>TFRQQTIDFLNDNIRRGIENYYDDLDFK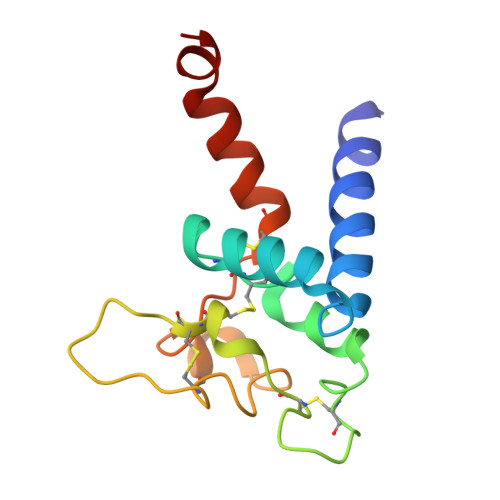NIMDFVQKKFKCCGGEDYRDWSKNQYHDCSAPGPLACGVPYTCCIRDTTEVVNTMCGYKTIDKERFSVQDVIYVRGCTNAVIIWFMDNLEVLFQ[24x]>[2x]MGHHHHHHEDRDPTQFEERHLKFLQQLGKGNFGSVEMCRYDPLQDNTGEVVAVKKLQHSTEEHLRDFEREIEILKSLQHDNIVKYKGVCYSAGRRNLKLIMEYLPYGSLRDYLQKHKERIDHIKLLQYTSQICKGMEYLGTKRYIHRDLATRNILVENENRVKIGDFGLTKVLPQDKEYYKVKEPGESPIFWYAPESLTESKFS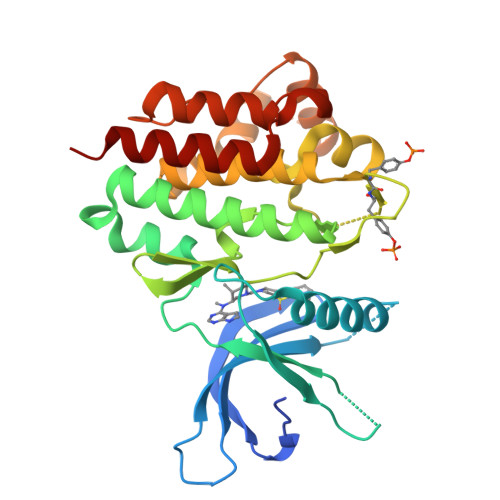VASDVWSFGVVLYELFTYIEKSKSPPAEFMRMIGNDKQGQSIVTHLIELLKNNGRLPRPDGCPDEIYMIMTECWNNNVNQRPSFRDLALRVDQVRDNMAG> PQPCLTGPRTCKDLLDRGHFLSGWHTIYLPDCRPLTVL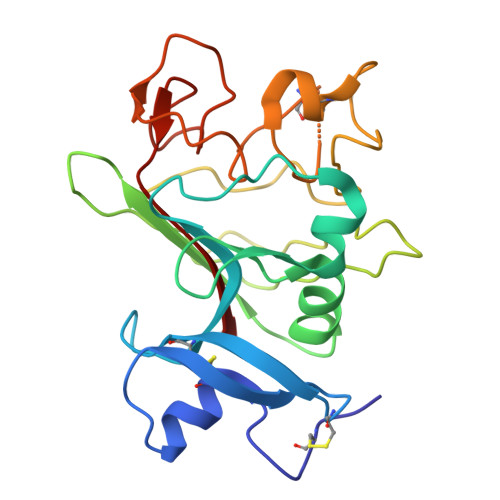CDMDTDGGGWTVFQRRVDGSVDFYRDWATYKQGFGSRLGEFWLGNDNIHALTAQGTSELRTDLVDFEDNYQFAKYRSFKVADEAEKYNLVLGAFVEGSAGDSLTFHNNQSFSTKDQDNDLNTGNCAVMFQGAWWYKNCHTSNLNGRYLRGTHGSFANGINWKSGKGYNYSYKVSEMKVRPA> MIKQRTLKNIIRATGVGLHSGEKVYLTLKPAPVDTGIVFSRTDLDPVVEIPARAENVGETTMSTTLVKGDVKVDTVEHLLSAMAGLGIDNAYVELSASEVPIMDGSAGPFVFLIQSAGLQEQEAA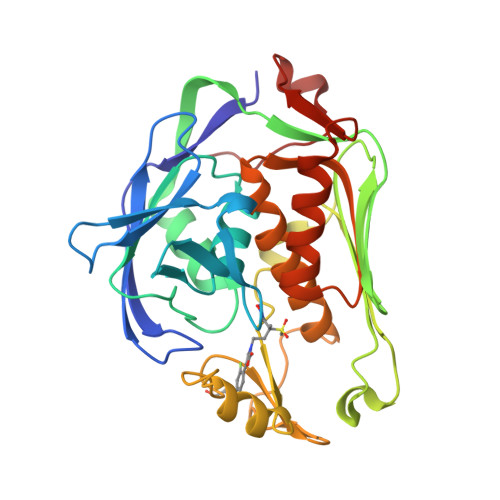KKFIRIKREVSVEEGDKRAVFVPFDGFKVSFEIDFDHPVFRGRTQQASVDFSSTSFVKEVSRARTFGFMRDIEYLRSQNLALGGSVENAIVVDENRVLNEDGLRYEDEFVKHKILDAIGDLYLLGNSLIGEFRGFKSGHALNNQLLRTLIADKDAWEVVTFEDARTAPISYMRP> MTTTESPT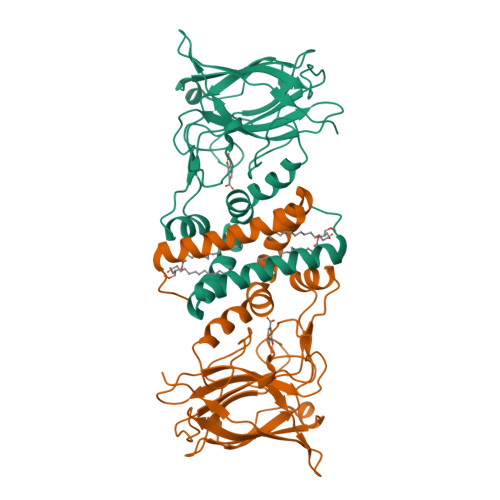AAGSGSAATDKFKAERATADTSPERLAAIAKDALGALNDVILKHGVTYPEYRVFKQWLIDVGEGGEWPLFLDVFIEHSVEEVLARSRKGTMGSIEGPYYIENSPELPSKCTDPMREEDEKITPLVFSGQVTDLDGNGLAGAKVELWHADNDGYYSQFAPHLPEWNLRGTIIADEEGRYEITTIQPAPYQIPTDGPTGQFIEAQNGHPWRPAHLHLIVSAPGKESVTTQLYFKGGEWIDSDVASATKPELILDPKTGDDGKNYVTYNFVLDPA> MVPISPIETVPVKLKPGMDGPKVKQWPLTEEKIKALVEICTEMEKEGKISKIGPENPYNTPVFACKKKDST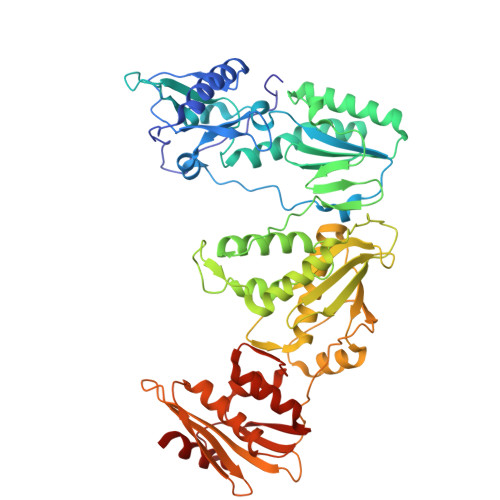KWRKLVDFRELNKRTQDFWEVQLGIPHPAGLKKKKSVTVLDVGDAYFSVPLDEDFRKYTAFTIPSINNETPGIRYQYNVLPQGWKGSPAIFQSSMTKILEPFKKQNPDIVIYQYMDDLYVGSDLEIGQHRTKIEELRQHLLRWGLTTPDKKHQKEPPFLWMGYELHPDKWTVQPIVLPEKDSWTVNDIQKLVGKLNWASQIYPGIKVRQLSKLLRGTKALTEVIPLTEEAELELAENREILKEPVHGVYYDPSKDLIAEIQKQGQGQWTYQIYQEPFKNLKTGKYARMRGAHTNDVKQLTEAVQKITTESIVIWGKTPKFKLPIQKETWETWWTEYWQATWIPEWEFVNTPPLVKLWYQLEKEPIVGAETFYVDGAANRETKLGKAGYVTNKGRQKVVPLTNTTNQKTELQAIYLALQDSGLEVNIVTDSQYALGIIQAQPDKSESELVNQIIEQLIKKEKVYLAWVPAHKGIGGNEQVDKLVSA>[2x]GPKFPRVKNWELGSITYDTLCAQSQQDGPCTPRRCLGSLMLPRKLQTRPSPGPPPAEQLLSQARDFINQYYSSIKRSGSQAHEERLQEVEAEVASTGTYHLRESELVFGAKQAWRNAPRCVGRIQWGKLQVFDARDCSSAQEMFTYICNHIKYATNRGNLRSAITVFPQRAPGRGDFRIWNSQLVRYAGYRQQDGSVRGDPANVEITELCIQHGWTPGNGRF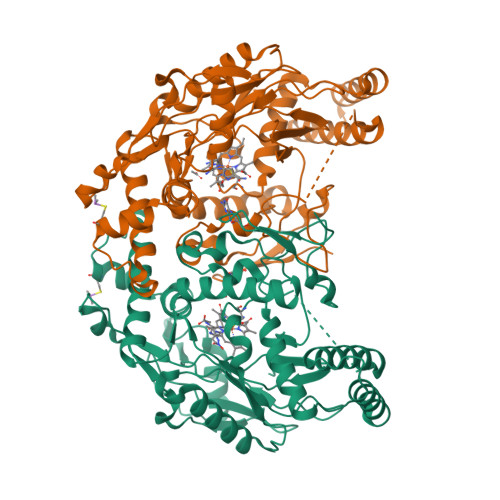DVLPLLLQAPDEAPELFVLPPELVLEVPLEHPTLEWFAALGLRWYALPAVSNMLLEIGGLEFSAAPFSGWYMSTEIGTRDLCDPHRYNILEDVAVCMDLDTRTTSSLWKDKAAVEINLAVLHSFQLAKVTIVDHHAATVSFMKHLDNEQKARGGCPADWAWIVPPISGSLTPVFHQEMVNYILSPAFRYQPDPW1-(pyridin-3-yl)-1,4-diazepane | C10 H15 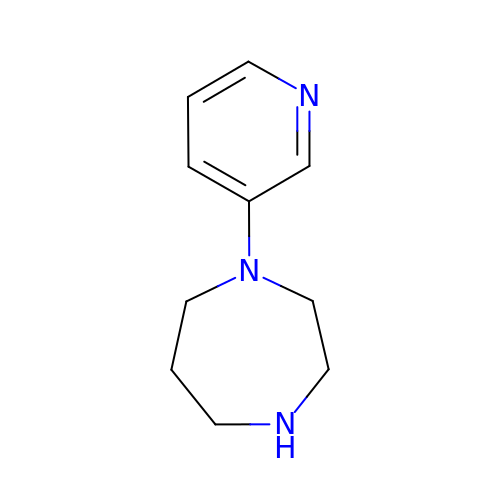N3 | JBOVXXZNZSULJJ-UHFFFAOYSA-N> GSHMVGDNKLDDKNIDKEKESSYRFPVIAMKVKKGI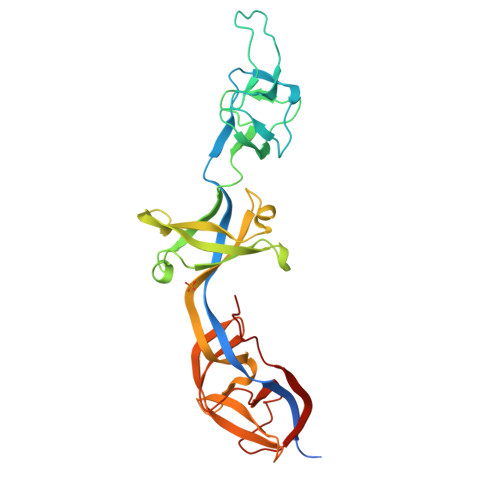LSDYLSLNGDVDTKVKADIFPDAVGKITSLRIKLGAYVQKGQIVATLDPSRPGSVYLKSPVRAPISGYILNITKKIGETVNPQSNIAVVGRIDTKQILTYVSEKYISNIKVGNDAIIEVGAYSNEKFKAKVSEISPILDSKSRTIEVYLTPIGSNLDKLIIGMFSKIKLITKRFKDVIKISREAVVEREGKKFVFKVDLESKSVQMLPITVLFEIDNIVALSGEVEENDLIVVEGMSALSNGSLINLVDTKEGLSAESNI>[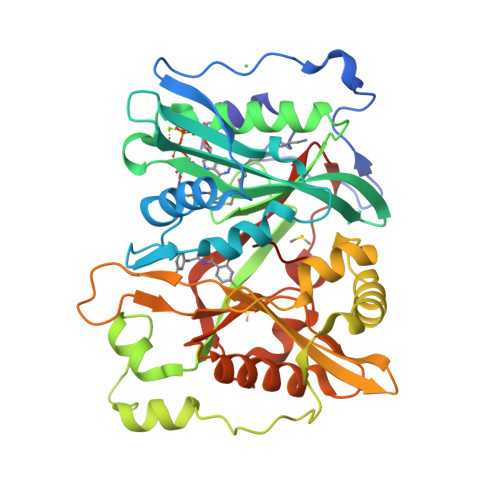3x]MDYKFWYTQPVPKINDEFNESVNEPFISDNKVEDVRKDEYKLPPGYSWYVCDVKDEKDRSEIYTLLTDNYVEDDDNIFRFNYSAEFLLWALTSPNYLKTWHIGVKYDASNKLIGFISAIPTDICIHKRTIKMAEVNFLCVHKTLRSKRLAPVLIKEITRRINLENIWQAIYTAGVYLPKPVSDARYYHRSINVKKLIEIGFSSLNSRLTMSRAIKLYRVEDTLNIKNMRLMKKKDVEGVHKLLGSYLEQFNLYAVFTKEEIAHWFLPIENVIYTYVNEENGKIKDMISFYSLPSQILGNDKYSTLNAAYSFYNVTTTATFKQLMQDAILLAKRNNFDVFNALEVMQNKSVFEDLKFGEGDGSLKYYLYNWKCASFAPAHVGIVLL> GSSMKASSGDQGSPPCFLRFPRPVRVVSGAEAELKCVVLGEPPPVVVWEKGGQQLAASERLSFPADGAEHGLLLTAALPTDAGVYVCRARN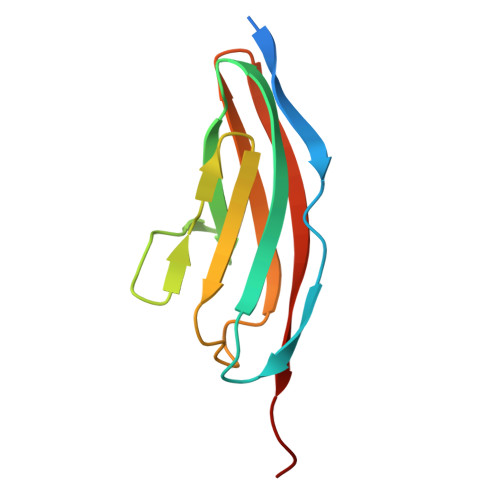AAGEAYAAAAVTVLEPPA>SISEKMVEALNRQINAEIYSAYLYLSMASYFDSIGLKGFSNWMRVQWQEELMHAMKMFDFVSRRGGRVKLYAVEEPPSEWDSPLAAFEHVYEHEVNVTKRIHELVEMAMQEKDFATYNFLQWYVAEQVEEEASALDIVEKLRLIGEDKRALLFL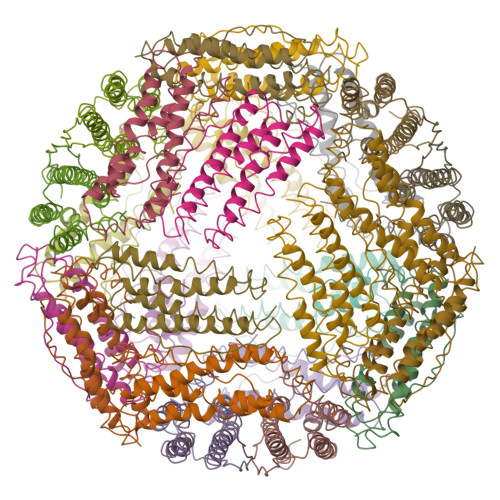DKELSLRQ[8x]> SMSAPAGEPPAPVRLRKNVCYVVLAVFLSEQDEV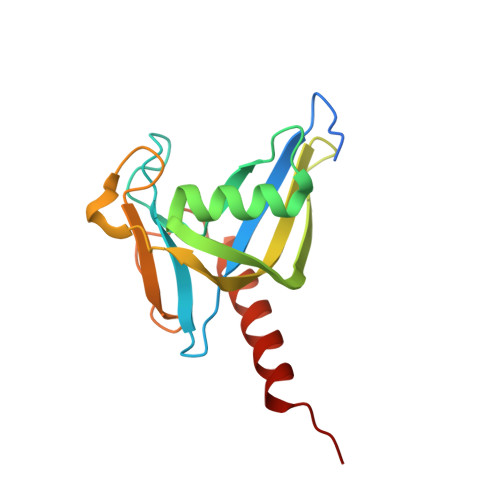LLIQEAKRECRGSWYLPAGRMEPGETIVEALQREVKEEAGLHCEPETLLSVEERGPSWVRFVFLARPTGGILKTSKEADAESLQAAWYPRTSLPTPLRAHDILHLVELAAQYRQQARHPLIL> QSSVGGCPVHRLAEDFDPFQDAYMADPAQFVRWAREQVPIFYAPKLNYWVVTRYDTIKQIFRDPVT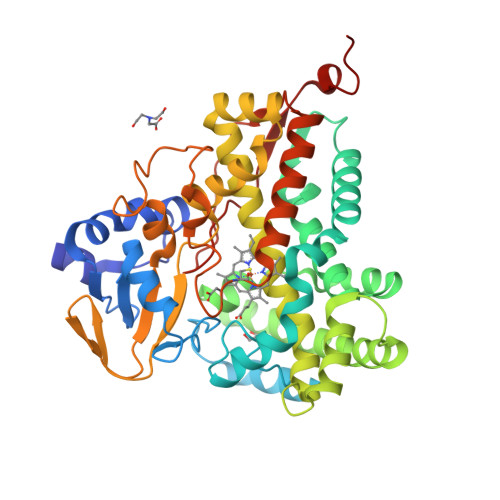FSPSNVLQSFAQPSAEVRQVLERYGYAFNRTLVNEDEPMHLERRRVLMEPFASEHLAEHEPMVRELVRRAVNRFIDTGRADLVDQMIWEVPFTVALHFLGVDDDDREKMRRFAIAHTVNAFGRPSPEEQLAVAETVGQFWQFCGEVLEKMRRTADGPGWMRYSIRQQKLYPDVVTDSYLHSMMQAIIVAAHETTVFATTNALKTLLEHETVWREICADPSLIPAAAEECLRYNGPVAGWRRRTTREVEVEGVRLPVGANILMVVASANHDSAHFDDPEFFDIGRSNASEHLNFGYGAHQCLGRNLGRMEMQIMIEELSRRLPHMRLAEQRFDYLHNVSFRAPRHLWVEWDPAQNPERRDP> GVSIRSMKNFYDWIKEFIRDQGEFIAQQSGWLELERSSYAKLIAQTISHVLNGGSLLVSADSSRHWFLNYILSNLNPKDLKERPLLSVIDFNASSFYPKNDANLSLATIEMTYQNPMFWHVGKIENEGLKTILLSKIPSFLWLFEELKEDCLLLKEHDSLLDYKLLQLFKLF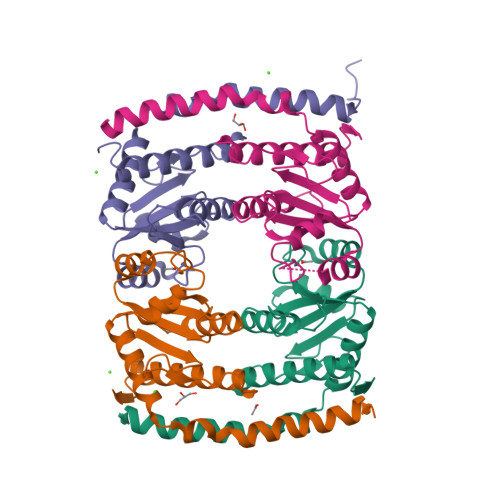ENALFSVLYNKVTL;>GVSIRSMKNFYDWIKEFVRDQGEFIAQQSGWLELERSSYAKLIAQTISHVLNGGSLLVSADSSRHWFLNYILSNLNPKDLKERPLLSVIDFNASSFYPKNDANLSLATIEMTYQNPMFWHVGKIENEGLKTILLSKIPSFLWLFEELKEDCLLLKEHDSLLDYKLLQLFKLFENALFSVLYNKVTL[3x]>MDYKDDDDKGENLYFQGSHNDKDLSTWQTFRRLWPTIAPFKAGLIVAGVALILNAASDTFMLSLLKPLLDDGFGKTDRSVLVWMPLVVIGLMILRGITSYVSSYCISWVSGKVVMTMRRRLFGHMMGMPVSFFDKQSTGTLLSRITYDSEQVASSSSGALITVVREGASIIGLFIMMFYYSWQLSIILIVLAPIVSIAIRVVSKRFRNISKNMQNTMGQVTTSAEQMLKGHKEVLIFGGQEVETKRFDKVSNRMRLQGMKMVSASSISDPIIQLIASLALAFVLYAASFPSVMDSLTAGTITVVFSSMIALMRPLKSLTNVNAQFQRGMAACQTLFTILDSEQEKDEGKRVIERATGDVEFRNVTFTYPGRDVPALRNINLKIPAGKTVALVGRSGSGKSTIASLITRFYDIDEGEILMDGHDLREYTLASLRNQVALVSQNVHLFNDTVANNIAYARTEQYSREQIEEAARMAYAMDFINKMDNGLDTVIGENGVLLSGGQRQRIAIARALLRDSPILILDEATSALDTESERAIQAALDELQKNRTSLVIAHRLSTIEKADEIVVVEDGVIVERGTHNDLLEHRGV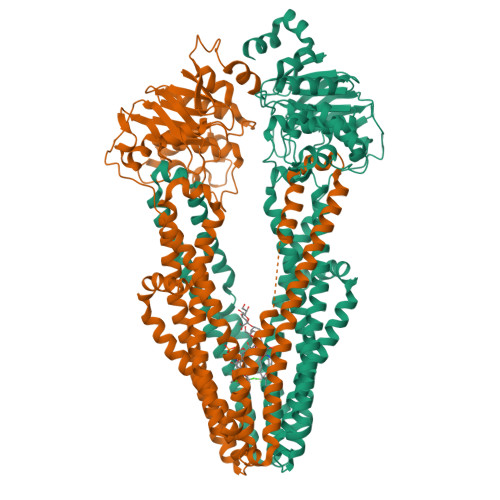YAQLHKMQFGQ[2x]> MGDHSQKDSPEDFIINRLSQALGIQKEKIKKSLETAQDDKGEVTNKDEFQGFIQQDNSTNILWVSGQSEKCTFYYGQLPPIDKFKKKGIAVIKLGLHKLTNENVAKDVVVVEITNNLLEHLNSVFNEIMSPVMQNPLNQQGWTDLVAKDLMEKFNNYVAQVYVLLGQIKGKTMLPLPSHKLTSSDTTPDKDKAHVFEGSIITWTKQIKNVLKLEPEQLLKYGNDPGPLAEIEFWQNKRDNLNLIDSQLKSVEVQNILHFLDNNKSTYTTPFTKLQAEVKKARLEANENYRYLFTLKDLFSKLQESQPSDFPTLYELFIPIMHTILLIYNKSKTYNQPPRLVVLIREICNAIISNAQAFVDKDTIFSLIDSKETTEACDKLQVTLDVCSKFKDAYFEYKAKAGGNWKLTSNALFVRLDSFLERCQDILHLTNTIVQFNKLEKIELGGTKGKTLTESIAQIFKEFEEAVQAFTSVSYDIMNIAEKKFDDDFYEFRSKIKELERRLASVITQGFDDYDTIYGRFKLLDNFEGLLTRPIIADELEKKHIVLLEMYKQDLKQVQSIFLEGKQFVDSMHENAPLFLNMPPIAGALTWCKSLRDRIQEPIEKLAQLGQGITEREEYKDVQKLYTSITKSIKDYEDQKILSWEKEVEDSSQDKLKQTLLCKDENDLIKVNFDPSLVRLLKEVKYFLLLRLEVPTTAKDIYTKAETYRTQIVALDMIVDNYNHIKTCLLPVEEPLVKKKIQDMEEEVKPGIEEIRWKSTNIDQFISKSKSIVDQLFETVNKMKDSLQKIHKSLANFNVKIIERKNRPMSPDDYDQFLKAIFSNKLTIVKDNGNQIQKLVKEVLDAVKADKKQNSWKNYNDYVNVIVIEGISTAIQTALLHLNEQINPVFIKRNDISPLFDIRLELGQSGIQFDPEIGESSNQLTVRNTIRNWINDFFNIAGTIQRLDTTMPGDFLQEIRSFFEIKQCLAMITQNLEWIENECNQFRARFDTYSYLWTEDEQISFNRFLDENEPKDEDGKGGDDDEGENTEKQNPLLKGCRAKIPNLDLFDEKITHLKAIQQEISRIKTPEDISWLRINLQPMKTALDARVTRWIRVYTDFLVNQFRTTQKNLLDFIEKTKDGIKKNPADHENLHDKKLLMSVMKVISDVKDVEPRREGIITRMKEMVTKLKKHNVPITEKGTDDPLQQIDNANSNFIEIYGRVFKVKADIIPLQAEETQNIKRDLDIFMKEVESFRKEFMQKLPFDYTESMGYENINNAYDTIMVYYHKLTAIEGRALEYNNLEKAFELQKSNYKQLKDCMNDLKNLKTMWDAIALIHFQYNDWKTKPWRQIKADILLDTNKTLGTQIKNLPKEIRNFKGYNVIVEKVKNMGTVLPLVSALHSEFMEDRHWSQLKQITGTVFDHNSLSFYFEDILALNLYKYENTVNEIVDVAQKEAKIEKKLKNIEQWWSKQVFEFTEYKETKTFASLDNMMEVLDQHSLDLMGMKSQGKYVEFFYDRVEDWREKLGRVDVVVNEWLKVQKNWKILYNIFLLSEDIRMQLPEDTKVFEGVDKEFKDMMSEVSANPSVVEACTIERRDVLVGWSQAIKKCEKALNDYLEQKKKSFPRFYFLSNQSLLTILSNGQNAPKVCEYLGDCFDGLKTLTFEPPANPAETSKVGIGMISKDDEKVPFSSKFICEGAVEHWLLNLEFRMRETLQEILEGAKNTADLWDSGDKPREEWVEGYNAQIALLTTTIVWTEDVGRAFEDLAGGSETAMKECQKLIEVRLENLIKKVRGDLHILERWKIINIITIDVHSRDVVEKFVIQKVSEAESFAWLSQLKFYWENKPDSDMHLRQTLRFPWEKDKNKNKCIIRIVDWFRFYSYEYIGNAIRLVITPLTDRCYITLTQALNLTMGGAPAGPAGTGKTETTKDLGRAIGIPVMVFNCSDQMNKDSMAQIFMGLSQSGAWGCFDEFNRISIEVLSVVSTQVKCVLDALKEKKTKFSFVEEGEIQLQDTVGFFITMNPGYAGRTELPENLKALFRSCAMVVPDLALICENMLMSEGFTMARVLSRKFVSLYMLSRELLSKQKHYDWGLRAVKSVLRQAGKLKRGDPDMPEDPLLMRALRDFNMPKIVTDDKVIFRRLIGDLFPKLDPPTKQNPELKKIVQDTTKKDMGLVAEELFVTKVVQLAEILEVRHCCFVIGPPGSGKTCVWKTLIKSYINSGEDAEYDTLNPKAVTSDELFGAYTKTKEWKNGVIAVIMKNQVKNEEKYKATHMHKWSVLDGDIDPEWIESLNTVMDDNKVLTLVSNDRIFLTPQMRLIFEISNLRNATPATVSRAGVLFINETDIGWMPYMNSWLERSQINILKQQKEMANMPEYPVIDDVAKSVFYRCFQSYFEQNIDVHDKNRVRHICPMVDIAMIQTICTILDALLIQHLPKLKQMKEEDEKQALEAFFIFAGLWAIGGPVGGGQDDSKDMKEFNTVWKGAAKVKFPEQGLCYDYYYDINENKWNTWKVEDYLPNDQPLFSKIYVATIHTTRLRYMIDIHLQRRKPILFIGSAGTGKTAVVRDYLNSTRPEQVSHKTINFSSFTDSLALQKNIESMVEKKNGRNYGSATNKVLICFIDDFNMPYVDKYGTQSPIQLLRLILDYGSIFNREQLEERKFLQDLLFFGCLNQKSGSFTVDLRLQRNFSVFSMYTPSSDVIKTIFGSILNAHLSTIDDKAQKMAFKLVEATYFTFDKILKNTTAFAPSAKRFHYQFNFRELARVCEGICRTTPGQYSGGDQGKLVRLWAHEMKRTFEDRFIANEHVEFFRRYLTEAISKCIGEFPETENPIAEPLIFTGFVAAHQGLDQQYTQCTIPVLKRVLDDKLEEYNEVKAQMNLVLFQQAMEHVSRICRILDMPGNNALLVGVGGSGKQSLCRLSTFINGFEIDQLVVTASFTINDLRNNLQEIYKKIAKPNSIARVFMITDSQIKEEQFLIPINDMLNSGWIFDLFPKEDMDSLVSGVRNEAKGEGVDVNNLTALTSYFLDKIRKNLKVVLCFSPVGDTMRIRSRKFPGIINNTSIDWFHPWPHEALIDVAFRFLEEIEFPTEEIRQSISLNMAKVHSSIDTANEKFLKLERRYNYTTPKSFLELIDFYKKLLTEKRETIQRQIQRYEMGLNILAETQNKVQGLQEELKVKMVEVNKQREETDILIEKVGKESALAEEEQTIANAEEEKTNVAAAEAEKISKEATEALAEALPALRSAEAAVDCLKKPHVTEMKNLGSPPAGVIVTARVVLILFNQGITLNDPDEKVWKKAVTFMNNPQAFIDKVKSFDGENIEPNIIEQSNKIIQDPSKKFNEKDMAGQSYAASKLCAWAVNIVTFNKIFKQVKPLQDAQKQANEILEEKKKELAIVKQRVAELNARVNSLKRQLEEAEARKMIVEQDAARCQSRLSAAENLVNGLAGENKRWTQNVKFLKENIKSMIGDSLLASAFVSYIGAFSAKLRLELWKNTWLPDIIEKGIPITEGIEPLKILTTEAIKSKWKNEGLPADPMSLENAAIITACARWPLIIDPQLQGSTWIRGKQGENLTTISLSQPKWLGALTSSISSGRAVLIEGIQQEIDATLDPLLQRAVKKNGNQLQLEIGGDPIDYDPNFKLFLMTKLINPHFRPEIAAQCTIINFIVTESGLEEQFIAMVVNIEKNELEMAKQDLVKKQNEYAVTLDKLESDLLQSLSEADPATILDNTELIQNLDKTKKTTIEITEQQQKAKVTEAEINIQREHYRVVAAEGSMLYFLVISLSVMDHMYQYSLESFITFFFKAINRTTVRDENRIPTLILNIRQTIYQWISRGLFEKHKLIFLTLIVFRLMQKKIIDVAYEVAEMDFLIKCPARPGVENTLDWLPNISWDQIQGLINLEEFRNFAHQLEKEAPNRFKDWYNELQPEDQKLPLDWKRLDSMPFKKLLVLRCLRPDRMTISLNNFIRAVLPQGDAFVEMDQKLAFSEILESVINEDAESTIPIFFILSPGSDPVKEVEKIAKKKRIEPGKNFFNIALGQGQDEIARRRIEEGNKEGHWVMLQNIHLMPTWLIELEKILDSYSGEAGGGNSEFRLFLSAEPSTGIPIGILDRSIKLTNEPPAGLKANMKRAWTYFSKEEIEDKDPKIKSILFALCFFHSTLIERRRFGPKGWNMSYPFNMGDLRDSYLVMNRYMEQNQGGKVPFNDLIYIFGEIMYGGHIVDDWDRRLCNSYLFNTMHEQLFDELELFPYIEG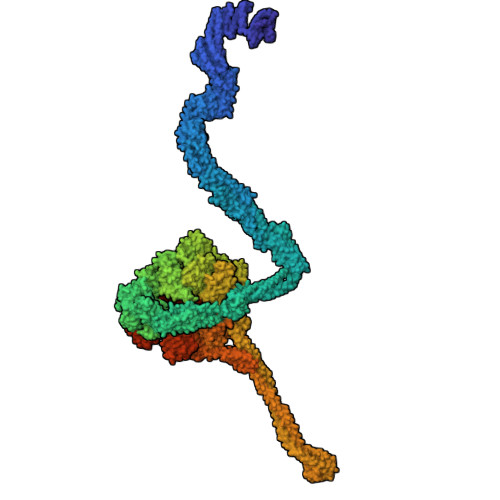KGLSFKVPGQNPYEKYIEHIETSLKQETPLAYGLHPNAEIGFRTDQCKTLFNTLLELMPKEQSRDEKSSDIKSSNEMASDLIKQLLEDSELKNKIFNMEEIKNKIDAENKGPYQNVFLQEIEYMNALLSEIVKDLEEIGQGLSGLLTVSENMEMIIESIALSRVPASWQKLAYPSKRGLQSWLANLFQRIEQLNIFRDDPYSIPRVVMISRFFNPQSFLTAIMQVISRAKAYELNKLYIQTEITKRSIEEIEGAAKEGAYVYGFILEGARWDYQLGQLEESKPKEMFSVLPVTYCKAIPLPPEGKEDKSLYQCPVYKTEDRGNTYVFTAQLKTRFPPRKWILAGVAIIMDVEGVSD>[2x]TVAYIAIGSNLASPLEQVNAALKALGDIPESHILTVSSFYRTPPLGPQDQPDAL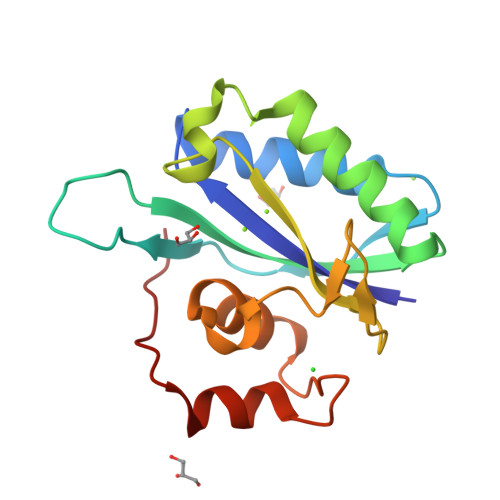NAAVALETSLAPEELLNHTQRIELQQGRVRKAERWGPRTLDLDIMLFGNEVINTERLTVPHYDMKNRGFMLWPLFEIAPELVFPDGEMLRQILHTRAFDKLNKW> MPRDNMASLIQRIARQASLTFRGSGGGRGASDRDAASGPEAPMQPGFPENLSKLKSLLTQLRAEDLNIAPRKATLQPLPPNLPPVTYMHIYETDGFSLGVFLLKSGTSIPLHDHPGMHGMLKVLYGTVRISCMDKLDAGGGQRPRALPPEQQFEPPLQPREREAVRPGVLRSRAEYTEASGPCILTPHRDNLHQIDAVEGPAAFLDILAPPYDPDDGRDCHYYRVL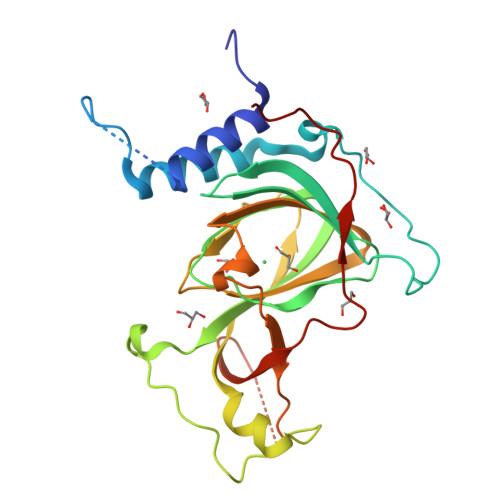EPVRPKEASSSASDLPREVWLLETPQADDFWCEGEPYPGPKVFP>MSEGPKKAGVLGSPIAHSRSPQLHLAAYRALGLHDWTYERIECGAAELPVVVGGFGPEWVGVSVTMPGKFAALRFADERTARADLVGSANTLVRTPHGWRADNTDIDGVAGALGAAAGHALVLGSGGTAPAAVVGLAELGVTDITVVARNSDKAARLVDLGTRVGVATRFCAFDSGGLADAVAAAEVLVSTIPAEVAAGYAGTLAAIPVLLDAIYDPWPTPLAAAVGSAGGRVISGLQMLLHQAFAQVEQFTGLP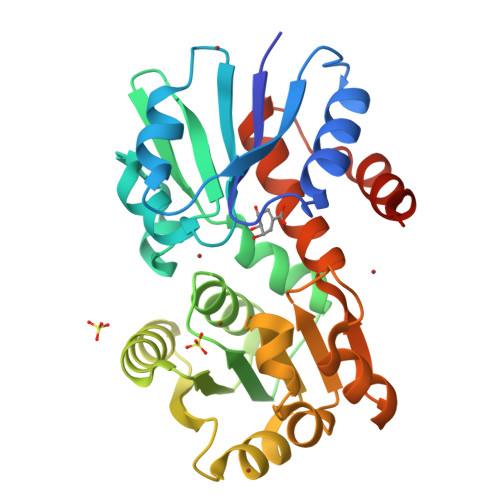APREAMTCALAALDLDHHHHHH[2x]>SLMADEIAKAQVARPGGDTIFGKIIRKEIPAKIIFEDDRCLAFHDISPQAPTHFLVIPKKHISQISVAEDDDESLLGHLMIVGKKCAADLGLNKGYRMVVNEGSDGGQSVYHVHLHVLGGRQMHWPPG[2x]

Diadenosine-5′,5-P1,P4-tetraphosphate (Ap4A) is a ubiquitous second messenger from bacteria to higher eukaryotes, which responds to environmental stresses and cell cycle phases. Ap4A then binds to the histidine triad nucleotide-binding protein 1 (HINT1), thereby disrupting the protein–protein interaction with microphthalmia-associated transcription factor (MITF), and the released MITF eventually promotes the transcription of mast cell activation genes. The HINT1 protein is a compact and symmetric dimer, with two adenosine pockets at opposite sides. Here we report that Ap4A specifically polymerizes HINT1 into (HINT1-Ap4A)n (HAn) filaments in solution and in the activated RBL cells.

To understand how Ap4A regulates HINT1, we set out to determine the crystal structure of human HINT1 in complex with Ap4A. HINT1 was reported to efficiently hydrolyze aminoacyl-adenylate (aa-AMP) and ADP, but neither ATP nor ApnA (such as Ap3A, Ap4A, and Ap5A). Incubation of 1 mM Ap4A with 25 μM HINT1 at 37 °C for 24 h showed minimal (<5%) hydrolysis. Therefore, we started with wild-type (WT) HINT1 to co-crystallize with Ap4A and solved the HINT1WT-Ap4A structure at a resolution of 1.52 Å. Consistent with previous reports, two HINT1 molecules formed a dimer through the five-stranded β-sheet and the central helix in the crystal structure. Despite having co-crystallized with different ligands, the three structures were nearly identical, with root mean square deviations (RMSDs) < 0.083 Å. However, in all the three structures, only the electron density corresponding to an AMP molecule was observed in the adenosine pocket, indicating that the ligands had been hydrolyzed by the HINT1WT protein during the crystallization, which took 3–7 days at 18 °C with a high protein concentration of ~2 mM.>[2x]EVKLILYHWTHSFSSQKVRLVIAEKALKCEEHDVSLPLSEHNEPWFMRL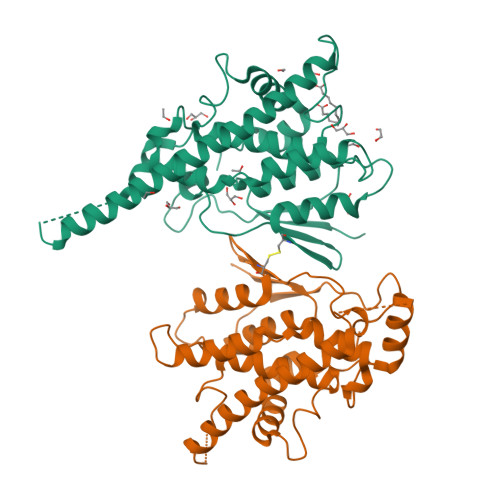NSTGEVPVLIHGENIICEATQIIDYLEQTFLDERTPRLMPDKESMYYPRVQHYRELLDSLPMDAYTHGCILHPELTVDSMIPAYATTRIRSQIGNTESELKKLAEENPDLQEAYIAKQKRLKSKLLDHDNVKYLKKILDELEKVLDQVETELQRRNEETPEEGQQPWLCGESFTLADVSLAVTLHRLKFLGFARRNWGNGKRPNLETYYERVLKRKTFNKVLGHVNNILIS>EDGYDMWLRYQPIADQTLLKTYQKQIRHLHVAGDSPTINAAAAELQRGLSGLLNKPIVARDEKLKDYSLVIGTPDNSPLIASLNLGERLQALGAEGYLLEQTRINKRHVVIVAANSDVGVLYGSFHLLRLIQTQHALEKLSLSSAPRLQHRVVNHWDNLNRVVERGYAGLSLWDWGSLPNYLAPRYTDYARINASLGINGTVINNVNADPRVLSDQFLQKIAALADAFRPYGIKMYLSINFNSPRAFGDVDTADPLDPRVQQWWKTRAQKIYSYIPDFGGFLVKADSEGQPGPQGYGRDHAEGANMLAAALKPFGGVVFWRAFVYHPDIEDRFRGAYDEFMPLDGKFADNVILQIKNGPIDFQPREPFSALFAGMSRTNMMMEFQITQEYFGFATHLAYQGPLFEESLKTETHARGEGSTIGNILEGKVFKTRHTGMAGVINPGTDRNWTGHPFVQSSWYAFGRMAWDHQISAATAADEWLRMTFSNQPAFIEPVKQMMLVSREAGVNYRSPLGLTHLYSQGDHYGPAPWTDDLPRADWTAVYYHRASKTGIGFNRTKTGSNALAQYPEPIAKAWGDLNSVPEDLILWFHHLSWDHRMQSGRNLWQELVHKYYQGVEQVRAMQRTWDQQEAYVDAARFAQVKALLQVQEREAVRWRNSCVLYFQSVAGRPIPANYEQPEHDLEYYKMLARTTYVPEPWHPASSSRVL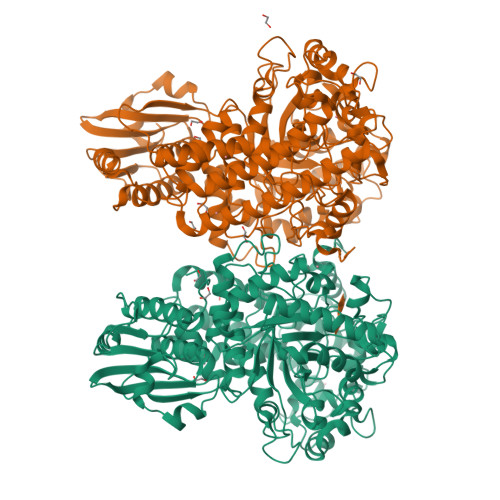K[2x]>GAMNNTIINSLIGGDDSIKRSNVFAVDSQIPTLYMPQYISLSGVMTNDGPDNQAIASFEIRDQYITALNHLVLSLELPEVKGMGRFGYVPY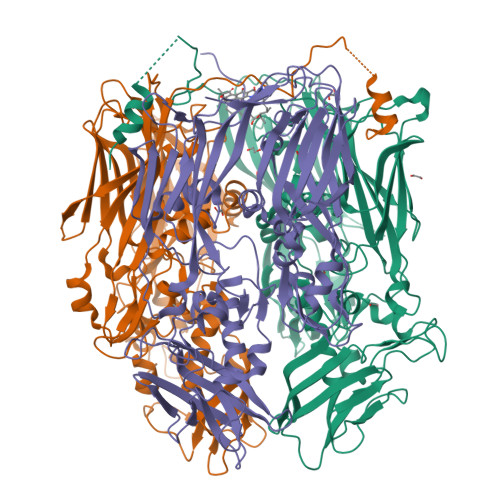VGYKCINHVSISSCNGVIWEIEGEELYNNCINNTIALKHSGYSSELNDISIGLTPNDTIKEPSTVYVYIKTPFDVEDTFSSLKLSDSKITVTVTFNPVSDIVIRDSSFDFETFNKEFVYVPELSFIGYMVKNVQIKPSFIEKPRRVIGQINQPTATVTEVHAATSLSVYTKPYYGNTDNKFISYPGYSQDEKDYIDAYVSRLLDDLVIVSDGPPTGYPESAEIVEVPEDGIVSIQDADVYVKIDNVPDNMSVYLHTNLLMFGTRKNSFIYNISKKFSAITGTYSDATKRTIFAHISHSINIIDTSIPVSLWTSQRNVYNGDNRSAESKAKDLFINDPFIKGIDFKNKTDIISRLEVRFGNDVLYSENGPISRIYNELLTKSNNGTRTLTFNFTPKIFFRPTTITANVSRGKDKLSVRVVYSTMDVNHPIYYVQKQLVVVCNDLYKVSYDQGVSITKIMGDNN[3x]>GSGETKVIYHLDEEETPYLVKIPVPAERITLGDFKSVLQRPAGAKYFFKSMDQDFGVVKEEISDDNARLPCFNG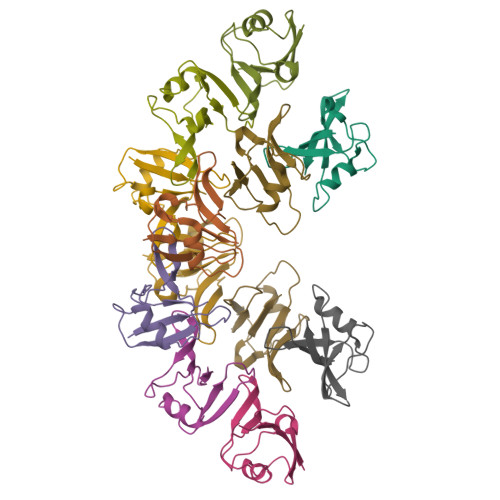RVVSWLVSS[12x]4-methyl-~{N}-(phenylmethyl)piperidine-1-carboxamide 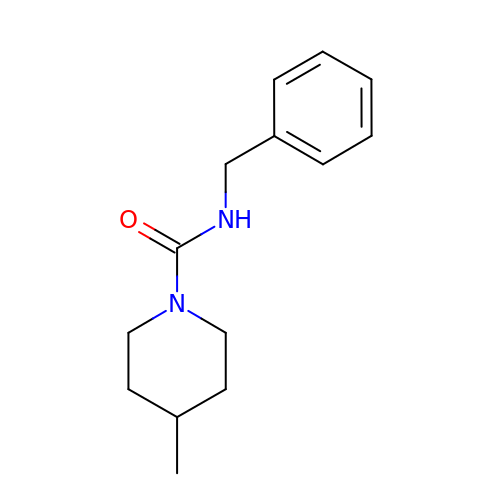| C14 H20 N2 O | ACFQCOHGQYWPEA-UHFFFAOYSA-N[(2R,3S,4S,5R,6R)-6-[(10E,12E,14E)-2,6,10,14,19,23-hexamethyl-25-(2,3,6-trimethylphenyl)pentacosa-6,8,10,12,14,16,18,20,22,24-decaen-2-yl]oxy-3,4,5-tris(oxidanyl)oxan-2-yl]methyl dodecanoate | C58 H86 O7 | 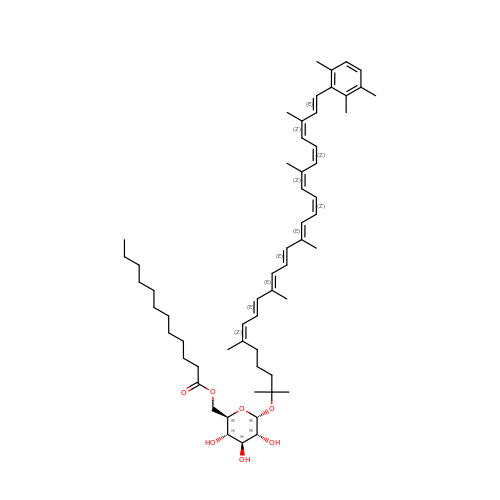NXEFUAFHBLRHFO-DDUHONCASA-N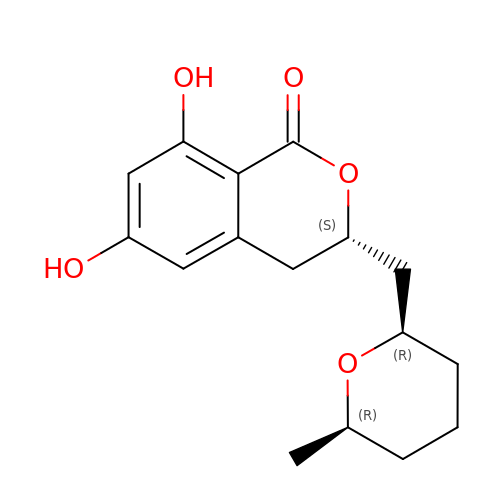(3S)-6,8-dihydroxy-3-{[(2R,6R)-6-methyloxan-2-yl]methyl}-3,4-dihydro-1H-2-benzopyran-1-one | C16 H20 O5 | WOMKDMUZNBFXKG-WQAKAFBOSA-N>MSELLIKNGKVFDPINGVKGDLMDIAIKDGKIVESVSSGAKVIDASGMTVMAGGVDAHSHIAGGKVNVGRIMRPDDGRSGLKPRTKITRPCSGYTVPNTFAMGYRYAELGYTTAFEAAIPILKARHTHEEFEDIPIIDKGGLTLFGSNWQVMDAVREGDLEKLAAYVAWGLRASRGYGVKIVNPGGGEAWGFGKNVRGLDDPVPGFDVTPSEIILALARANEMLNLPHSIHLHCNRLGTPGNYETTIETMRRLEKIKPSRDRQVVHVTHVTFNAWGGTHFGNFESKADAVAEYLNKSDHVTIDMGQLIFGNATTMTADGPVQYANARLLGAKWGNGDVELEDASGVVPLFYMRKMYVHDIMWAIGLELALLTNDPWQVLLTTDHPNGGPFVNYPEVIALLMSAKKREEEIAKLSDKMQERTCLSGIDREFDWYDIAIKTRAAHAKILGLHEYGKGHLGVGADGDVTIYNINTESVDPSVEHAAVKKAFQLPAYTIKGGEIVAKEGEITATPTGRTFWVDARVPEEYTTRMMKDLEWKFRKYYSVKMANYMVQDEYVQHPVVLEAGVN[2x];>[2x]MVEITDAICSFCGSLCDDLTVKVEDNRIVDVRRACRLGAKKILGHERIPAPMIRDGSGELVEASYDEAIDRAAEILAGSKRPLLYGWASTSCEAQSKGILLAEIIGGVIDNTASVCHGPSTLAVQEKGLPTASLGQMKNRADLVIFWGCNPVHAHPRHMSRYSVYKKGFFLDRGRQNRKFVTVDVRMTDTAAISDEFIQIEQGSDYLIVSAIRALVNGKGDVVPETVAGVPKEELARVAEMMTSCRFGMILYGMGLTQSRSKYKNIDIALSLINDLNTKTKFVITPMRGHYNVTGFGQVCSWQTGFPTVDLARGVPYYNPGEMSANDLLMRDEVDSAMIIAGDAGAHFPAASIRNLAKVPLVQIDPYPNATTELANVVIPAAIVGIECEGTAYRMDGVSLRMRKLVESDYLSDEEILDRIIEKVRVIKGE;>[2x]MQTVTLTPRKSSKISVEAETITPDNFAGKTVEEIEKVTVWEGNNKTTLGEFFEVALDGSDTPENTKIVIEGSIPRVKRVGEGMSAGIILINGDVDMHVGAKMRGGRITVKGNADSWAGREMKGGELIIEGNAEYYLGAGYRGESCGMRGGRITVFGNARDYVGEHMCGGEIIIKGNAGLMPGISNNGGKIIIEGNTTMPGGEMKKGTIIINGRVDELVPVYQQEEDEELDGVSYKKYTGDVVAGGKGTLYIKA;>MKRDVNIVTGRTIKQGADIENKLSREYFEACARCEVGPEDLRALGISEGSNVRISTDFGSVVVPVALCEGNPTGIVFIPMGPWANAVVNPDTHGCGMPGFKGVPGTIEPTDDTPLDLKSLMKLYKE[2x];>MMNGYDQLVEEVIDAGICVSCGNCAAVCPLQYISMEEKKPVQDREKRDEIEKRSGLACNDCNLCAMSCPRIEPTYFWQKRELKRMEHEGEVKAARTTYKPIQDVCQDGGIVTTLFKYLLDSGRVDGVVVSQYNGDYNPVPVLAKREDDLLRAAGTRYTVSPAYSPLTDIKQLKDDGYERIAIVGTPCQIYALRKTQAIYNSQRLLIPHNIITFAIGLFCAEEFDDRILQDLEVDIADVTGFDVKKEGLIISLKSGEKKIIPHEDLEEYVREGCKICSDFNSPYADISVGSVGSPPGWSTVIVRTETGREIYQKLLEKGLIEETTVDEKGLKLIDKMAQKKINNAQTKIKERSNKESEEE[2x];>[2x]MANQMSFKKVKVSEECVGCGVCETVCPVNNLLEDGAEFDPDRAKLAIKVTNGEAAVDEEVCLTCGTCTFNCPSGAVYAEYEPRAS

Here, we study the molecular basis of the CO2-generating steps of anaerobic ethane oxidation by characterising native enzymes of the thermophile Candidatus Ethanoperedens thermophilum obtained from microbial enrichment. We perform biochemical assays and solve crystal structures of the CO dehydrogenase and formylmethanofuran dehydrogenase complexes, showing that both enzymes deliver electrons to the F420 cofactor. Both multi-metalloenzyme harbour electronic bridges connecting CO and formylmethanofuran oxidation centres to a bound flavin-dependent F420 reductase. Based on the crystal structures, enzymatic activities, and metagenome mining, we propose a model in which the catabolic oxidising steps would wire electron delivery to F420 in this organism.

The crystal structure of the Fmd/Fwd complex from Ca. E. thermophilum was refined at a resolution of 1.97 Å. Compared to the initial prediction of a molybdenum-containing enzyme, the anomalous data confirmed the presence of a tungsten atom in the active site, therefore renaming the complex Fwd. The Fwd complex forms a heterohexameric assembly in which the canonical polyferredoxin FwdF subunit is replaced by an F420-reductase module (CAD7775209, named FwdI). As FwdF was reported to be required for large Fmd/Fwd-containing complexes or supercomplexes, its substitution by the FwdI subunit prevents the formation of higher oligomeric states. The resulting Fwd complex is consequently the smallest ever structurally described. FwdI shares a similar organisation and (metallo)-cofactor content to the ζ subunit of ACDS, with the exception of the absence of the C-terminal extension involved in dimerisation. The six [4Fe-4S] clusters dispatched in FwdBGI would allow an efficient electron transfer between the tungstopterin to the FAD of FwdI, therefore possibly coupling formate oxidation to F420-reduction.>[3x]GHMSMQGPRTRPRKPIRAGEVLFAVGGWASGDAISSVERYDPQTNEWRMVASMSKRRCGVGVSVLDDLLYAVGGHDGSSYLNSVERYDPKTNQWSSDVAPTSTARTSVGVAVLGGFLYAVGGQDGVSALNIVERYDPKENKWTRVASMSTRRLGVAVAVLGGFLYAVGGSDGTSPLNTVERYNPQENRWHTIAPMGTRRKHLGCAVYQDMIYAVGGRDDTTELSSAERYNPRTNQWSPVVAMTSRRSGVGLAVVNGQLMAVGGFDGTTYLKTIEVFDPDANTWRLYGGMNYRRLGGGVGVIKMTHAE;> GHMSMQGPRTRPRKPIRAGEVLFAVGGWASGDAIS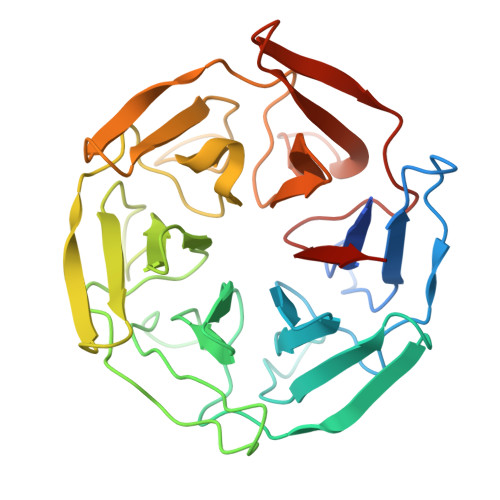SVERYDPQTNEWRMVASMSKRRCGVGVSVLDDLLYAVGGHDGSSYLNSVERYDPKTNQWSSDVAPTSTARTSVGVAVLGGFLYAVGGQDGVSALNIVERYDPKKNKWTRVASMSTRRLGVAVAVLGGFLYAVGGSDGTSPLNTVERYNPQENRWHTIAPMGTRRKHLGCAVYQDMIYAVGGRDDTTELSSAERYNPRTNQWSPVVAMTSRRSGVGLAVVNGQLMAVGGFDGTTYLKTIEVFDPDANTWRLYGGMNYRRLGGGVGVIKMTHAE;> GHMSMQGPRTRPRKPIRAGEVLFAVGGWASGDAISSVERYDPQTNEWRMVASMSKRRCGVGVSVLDDLLYAVGGHDGSSYLNSVERYDPKTNQWSSDVAPTSTARTSVGVAVLGGFLYAVGGQDGVSALNIVERYDPKENKWTRVASMSTRRLGVAVAVLGGFLYAVGGSDGTSPLNTVERYNPEENRWHTIAPMGTRRKHLGCAVYQDMIYAVGGRDDTTELSSAERYNPRTNQWSPVVAMTSRRSGVGLAVVNGQLMAVGGFDGTTYLKTIEVFDPDANTWRLYGGMNYRRLGGGVGVIKMTHAE> GLPTVLTPGSEQFLTTDDRQSPSAMPNYEPTPLIHIPGEVKNLLEIAQVDTLIPLNNTTNTTGLGMYRIPLVQNMQGEQVFGFRLYLGDGVLKTTLLGELCQYFTHWAGSLRLSFMYTGPALSSAKLLIAYTPPGAQGPTKRKEAMLGTHVVWDIGLQSTVVLNIPWTSGVQYRYTDPDTYTSAGFVSCWYQTSLVLPPQTQQTVYMLGFISACPDFKLRLMKDTQSI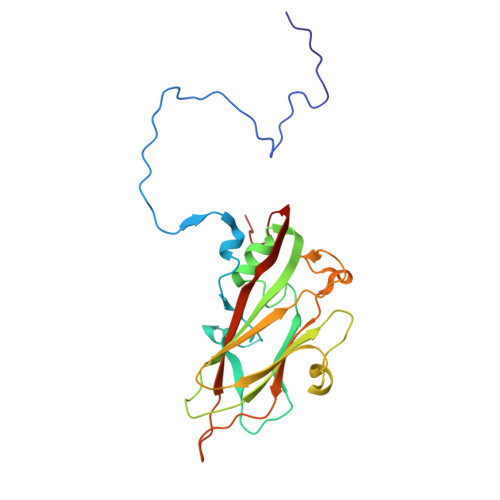HQ> ETEYVRRFHRHEPRDHQCSSAVAKHIKAPVHLVWSLVRRFDQPQLFKPFVSRCEMKGNIEIGSVREVNVKSGLPATRSTERLELLDDNEHI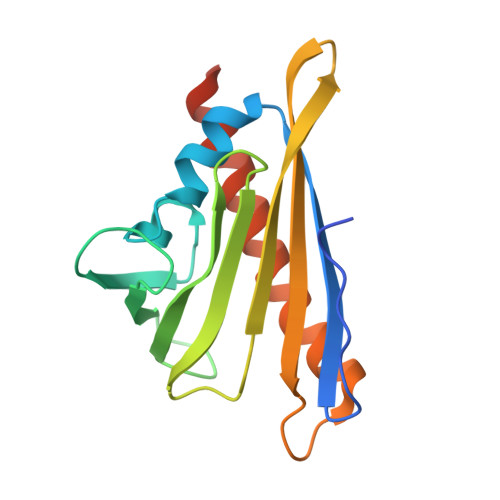LSVRFVGGDHRLKNYSSILTVHPEVIDGRPGTLVIESFVVDVPEGNTKDETCYFVEALLKCNLKSLAEVSERLVVKDQTEPLDR>[2x]DAGTPTDAGTPTDAGTPTDAGTPTDAGTQVPWSNVKSFTYQLTNYPQGKLDAIAASKFDLAIVELVRDGSSGYFTAAEISALKARGKQVLAYFEIGAIEEYRPEWSQVPADLKLGPVSGWPDEQYVKYWDERWWPIVQGRIDRALAAGFNGCYLDMVVTYEEIPANSAG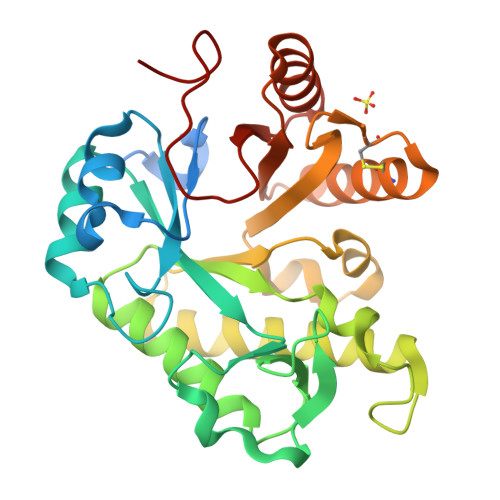TNRADLARKMVALIARINTYAKARNPDFKVVPQNSPELVDDPAYLPAIDGLGMEDMYWSDDVACDEGWCEENRTNAARVRAAGKLVLSTDYATQSAHVADAYTRSRAAGFVPYVTVRALDRVTVNAGWDPQ4-[5-chloro-3-(1-methylethyl)-1H-pyrazol-4-yl]-N-(5-piperazin-1-ylpyridin-2-yl)pyrimidin-2-amine 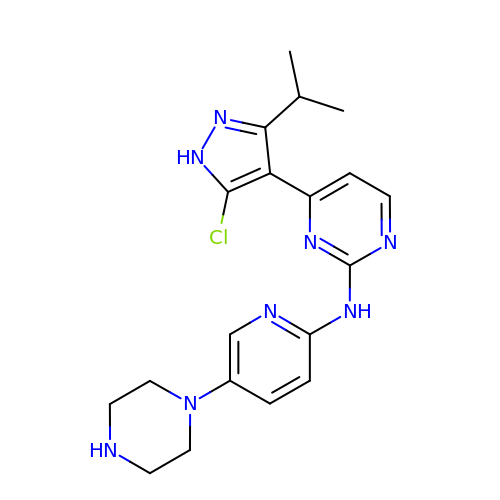| C19 H23 Cl N8 | ZGJLAVYYTJNBMN-UHFFFAOYSA-N> GPGSMGGLLTDKVVVISGVGPALGTTLARRCAEQGADLVLAARTVERLEDVAKQVTDTGRRALSVGTDITDDAQVAHLVDETMKAYGRVDVVINNAFRVPSMKPFANTTFEHMRDAIELTVFGALRLIQGFTPALEESKGAVVNVNSMVVRHSQAKYGAYKMAKSALLAMSQTLATELGEKGIRVNSVLPGY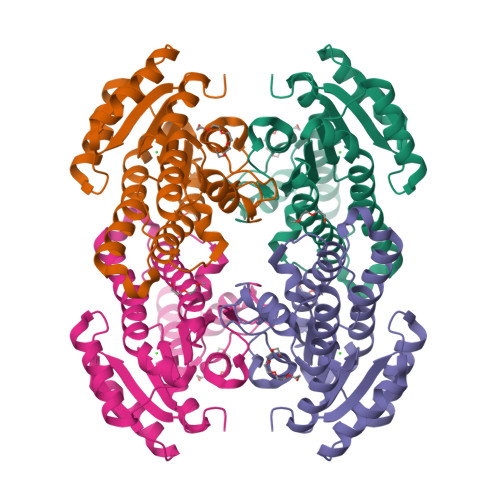IWGGTLKSYFEHQAGKYGTSVEDIYNAAAAGSDLKRLPTEDEVASAILFMASDLASGITGQALDVNCGEYKA N~2~-ACETYL-L-GLUTAMINE 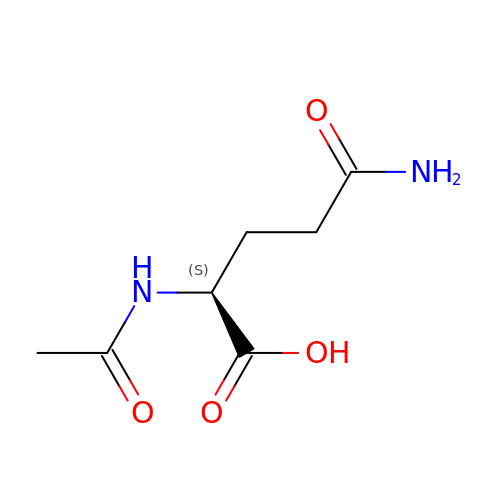| C7 H12 N2 O4 | KSMRODHGGIIXDV-YFKPBYRVSA-N>DPSSRSTRKAVIGYYFIPTNQINNYTETDTSVVPFPVSNITPAKAKQLTHINFSFLDINSNLECAWDPATNDAKARDVVNRLTALKAHNPSLRIMFSIGGWYYSNDLGVSHANYVNAVKTPASRAKFAQSCVRIMKDYGFDGVDIDWEYPQAAEVDGFIAALQEIRTLLNQQTITDGRQALPYQLTIAGAGGAFFLSRYYSKLAQIVAPLDYINLMTYDLAGPWEKVTNHQAALFGDAAGPTFYNALREANLGWSWEELTRAFPSPFSLTVDAAVQQHLMMEGVPSAKIVMGVPFYGRAFKGVSGGNGGQYSSHSTPGEDPYPSTDYWLVGCEECVRDKDPRIASYRQLEQMLQGNYGYQRLWNDKTKTPYLYHAQNELFVTYDDAESFKYKAKYIKQQQLGGVMFWHLGQDNRNGDLLASLDRYFNAADYDDSQLDMGTGLRYTGVGPGNLPIMTAPAYVPGTTYAQGALVSYQGYVWQTKWGYITSAPGSD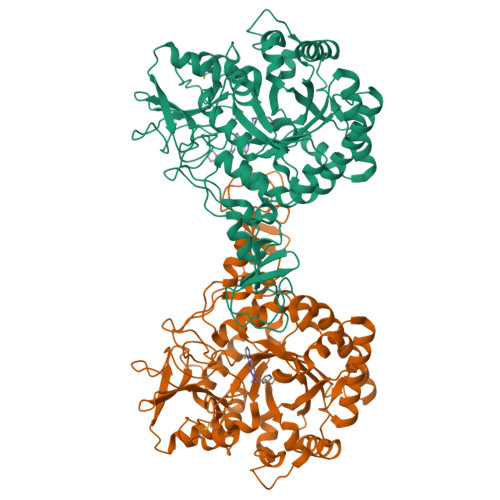SAWLKVGRVAHHHHHH[2x]>[2x]MRGSHHHHHHGSMIFSSISIIRTFMGFAGHGTAGGIIGLFTEVLRLLWPNKQNDLWESFMNEVEALINQEITEAVVSKALSELEGLRNALEGYTSALEAWQNNRSDKLKQLLVYERFVSTENLFKFAMPSFRSVGFEGPLLTVYAQAANLHLFLLKNAELFGAEWGMQQYEIDLFYNEQKGYVEEYTDHCVKWYKEGLNKLKNASGVKGKVW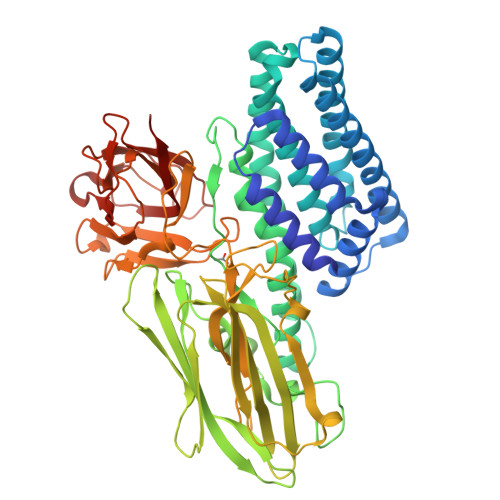ENYNRFRREMTIMVLDLLPLFPIYDARTYPMETVTELTRQIFTDPIGLTGINETKYPDWYGAASSEFVLIENRAIPKPGLFQWLTKINVRARVVEPNDRFAIWTGHSVVTQYTKSTTENTFNYGTSSGSTLSHTFDLLSKDIYQTYSIAAANKSATWYQAVPLLRLYGINSSNVLSEDAFSFSNNIPSSKCKSTYSSDQLPIELLDEPIYGDLEEYGHRLSYVSEIFKETGSGTIPVLGWTHVSVRPDNKLYPDKITQIPAVKAFETNTAGVEIIDSASTGGPILKIVNNNLPSNQVFRMRLSFSEPQKIKVRVRYAATGDGVMSFSGIAHDEYFTATMKEGEALKYSYLTMGNDYAGTAAELSMLYIIKANTSNCTIYIDKIEFIPVVDLQPSLIS> AHFEAYSLSDNDYDGIKKLLQQLFLKAPVNTAELTDLLIQQNHIGSVIKQTDVSEDSNDDMDEDEVFGFISLLNLTERKGTQCVEQIQELVLRFCEKNCEKSMVEQLDKFLNDTTKPVGLLLSERFINVPPQIALPMYQQLQKELAGAHRTNK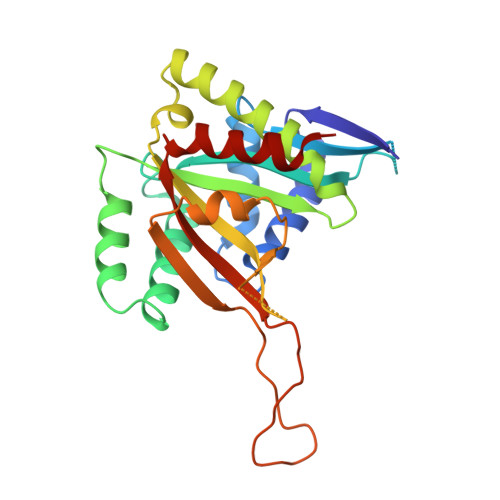PCGKCYFYLLISKTFVEAGKNNSKKKPSNKKKAALMFANAEEEFFYEKAILKFNYSVQEESDTCLGGKWSFDDVPMTPLRTVMLIPGDKMNEIMDKLKEYLSV>KPIEIIGAPFSKGQPRGGVEKGPAALRKAGLVEKLKETEYNVRDHGDLAFVDVPNDSPFQIVKNPRSVGKANEQLAAVVAETQKNGTISVVLGGDHSMAIGSISGHARVHPDLCVIWVDAHTDINTPLTTSSGNLHGQPVAFLLKELKGKFPDVPGFSWVTPCISAKDIVYIGLRDVDPGEHYIIKTLGIKYFSMTEVDKLGIGKVMEETFSYLLGRKKRPIHLSFDVEGLDPVFTPATGTPVVGGLSYREGLYITEEIYK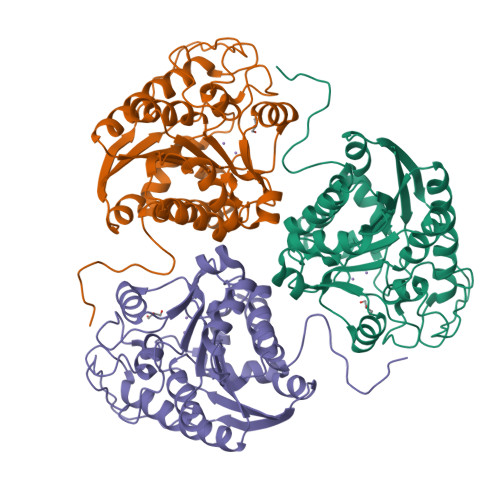TGLLSGLDIMEVNPTLGKTPEEVTRTVNTAVALTLSCFGTKREGNHKPETDYL[3x]>MSKLPFLSRAAFARITTPIARGLLRVGLTPDVVTILGTTASVAGALTLFPMGKLFAGACVVWFFVLFDMLDGAMARERGGGTRFGAVLDATCDRISDGAVFCGLLWWIAFHMRDRPLVIATLICLVTSQVISYIKARAEASGLRGDGGFIERPERLIIVLTGAGVSDFPFVPWPPALSVGMWLLAVASVITCVQRLHTVWTSPGAIDRMAIPGKGDRENLYFQ[2x]

One such potential target is the mycobacterial phosphatidylinositol phosphate synthase (M. tuberculosis PgsA1). PgsA1 catalyzes the conjugation of the 1’ hydroxyl group of D-myo-inositol-3-phosphate (ino-P) with a lipid tail of an acceptor substrate, cytidine diphosphate diacylglycerol (CDP-DAG), forming phosphatidylinositol phosphate (PIP). 1 D-myo-inositol-3-phosphate+CDP-DAG→PIP+CMP 2 PIP→PI+Pi PgsA1 belongs to the class I CDP-alcohol phosphotransferases (CDP-APs), integral membrane proteins that catalyze the formation of a phosphodiester bond to merge a CDP-alcohol and a second alcohol, releasing cytidine monophosphate (CMP). The M. tuberculosis PgsA1 was identified as a promising candidate for drug development, due to its essential role in growth and proliferation of the pathogen and differences between the Eukaryotic and mycobacterial PI biosynthesis pathways.

To unambiguously assign the metal-binding geometry we also determined the structure of the Mn2+—substituted protein to 1.88 Å resolution, allowing X-ray anomalous dispersion identification of the metal binding positions. The Mn2+ substituted crystals diffracted to 1.88 Å and belonged to space group P212121 with one homodimer per asymmetric unit as for the apo structure. As expected, our metal-substituted structure reveals a di-nuclear metal binding site coordinated by D68, D71, D89, and D93 of the conserved sequence motif, as indicated by two clear peaks within a metal coordinating distance to the chelating carboxylate side chains. In chain B of the M. tuberculosis PgsA1 homodimer, however, the anomalous difference density, corresponding to the aspartate-chelated Mn-ions, is extended indicating two alternate binding positions for the metal ion in site 2 (indicated as 2a and 2b in Fig. 1d, e). Besides the anticipated protein-bound metal ions, additional anomalous difference density peaks were found: two in chain A and one in chain B. These additional Mn-ions appeared to be coordinated by serendipitously bound citrate molecules, most likely derived from the crystallization condition. Two citrate molecules are chelating two Mn-ions in chain A and one citrate molecule is found chelating one Mn ion in chain B. The citrate-Mn complex is most likely not biologically relevant and result from the presence of 100 mM citrate and 120 mM Mn2+ in the crystallization solution. The presence of the metal ions and bound Mn-citrate ligand complexes in both protein chains appear to have a stabilizing effect on the N-terminal helix and C-terminal loop which now can be indubitably traced in the electron density. In the Mn-citrate complex structure one of the citrate carboxylates assumes the position of SO42− (1) in both protein chains. However, the Mn-citrate complex revealed a plausible binding pocket for this substrate.The alkaline α-galactosidase AtAkαGal3 from Arabidopsis thaliana catalyzes the hydrolysis of α-d-galactose from galacto-oligosaccharides under alkaline conditions. Here, thin-layer chromatography is used to demonstrate that AtAkαGal3 exhibits a dual function and is capable of synthesizing stachyose using raffinose, instead of galactinol, as the galactose donor. The structure of AtAkαGal3 comprises three domains: an N-terminal domain with 13 antiparallel β-strands, a catalytic domain with an (α/β)8-barrel fold and a C-terminal domain composed of β-sheets that form two Greek-key motifs. A sequence comparison of AtAkαGal3 with acidic α-galactosidases further confirmed that Asp383 and Asp447 are presumably critical residues that serve as the nucleophile and the catalytic acid/base, respectively.

The crystal structure of D383A in complex with raffinose was determined at a resolution of 2.47 Å. Lys75, Tyr78, Asp446 and Tyr449 help to stabilize the glucose moiety of the raffinose substrate at the +1 subsite. The NE1 group of Trp78 and OD1 of Asp446 form hydrogen bonds to O4 of the hydroxyl group with distances of 3.08 and 3.47 Å, respectively. NZ of the Lys75 side chain stabilizes O3 of the hydroxyl group through a hydrogen bond with a distance of 3.54 Å. Tyr449 stabilizes the glucose at the +1 subsite and the fructose moiety at the +2 subsite of raffinose via hydrogen bonds from its side-chain OH group to the O3 hydroxyl groups of both galactose and fructose with distances of 3.52 Å. One water molecule that forms a hydrogen bond (distance of 2.70 Å) to the side chain of Asp447 seems to be involved in stabilization of the fructose moiety through weak hydrogen bonding. The interactions of the residues at the −1 subsite with the galactosyl moiety of raffinose are similar to those with the galactosyl moiety of galactinol bound in the D383A complex. Our crystal structures of wild-type AtAkαGal3 and its D383A mutant in complex with galactose and with hydrolyzed raffinose, i.e. galactose and sucrose, reveal one water molecule at the conserved position near the anomeric C atom and Asp447. This water is replaced by O4 of galactose in the +1 subsite of raffinose and stachyose in the complexes of D383A with raffinose and stachyose.

>MTIKPAVRISDGNLIIKNRTILTGVPDNVITTSASEAGPVEGVFVGAVFNKEESKHIVPIGTLRNSRFMSCFRFKLWWMAQRMGEMGRDIPYETQFLLVESNDGSHLESDGANGVECNQKVYTVFLPLIEGSFRSCLQGNVNDEVELCLESGDVDTKRSSFTHSLYIHAGTDPFQTITDAIRTVKLHLNSFRQRHEKKLPGIVDYFGWCTWDAFYQEVTQEGVEAGLKSLAAGGTPPKFVIIDDGWQSVERDATVEAGDEKKESPIFRLTGIKENEKFKKKDDPNVGIKNIVKIAKEKHGLRYVYVWHAITGYWGGVRPGEEYGSVMKYPNMSKGVVENDPTWKTDVMTLQGLGLVSPKKVYKFYNELHSYLADAGVDGVKVAVQCVLETLGGGLGGRVELTRQFHQALDSSVAKNFPDNGCIACMSHNTDALYCSKQAAVIRASDDFYPRDPVSHTIHIASVAYNSVFLGEFMQPDWDMFHSVHPAAEYHASARAISGGPLYVSDSPGKHNFELLRKLVLPDGSILRARLPGRPTRDCLFADPARDGVSLLKIWNMNKYTGVLGVYNCQGAAWSSTERKNIFHQTKTDSLTGSIRGRDVHSISEASTDPTTWNGDCAVYSQSRGELIVMPYNVSLPVSLKIREHEIFTVSPISHLVDGVSFAPIGLVNMYNSGGAIEGLRYEAEKMKVVMEVKGCGKFGSYSSVKPKRCVVESNEIAFEYDSSSGLVTFELDKMPIENKRFHLIQVEL[2x]> RTEPVSTTISKSFFAPEPQIQPSFGKNVGKEGGLLFSVSLTVPENVSQVTVYP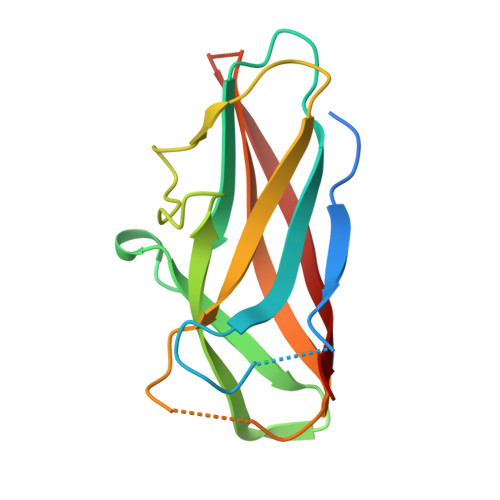VYDEDYGLGRLVNTADDSQSIIYQIVDDKGRKMLKDHGAEVTPNQQITFRALNYTSGDKEIPPGIYNDQVMVGYYVNDNKQRTEIATKNFPVSTTIS> AAEPASRNVPFPYAETDVADLQARMTAGELDSTTLTQAYLQRIAALDRTGPRLHAVIELNPDALKEAAERDRERRDGRLRGPLHGIPLLLKDNINAAPMATSAGSLALQDFRPDDAYLVRRLRDAGAVVLGKTNLSEWMNFRSNNSISGWSARGGQTRNPYRPSHSPCGSSSGSAVAVAANLASVAIGTETDGSIVCPAAINGVVGLKPTVGLVSRDGI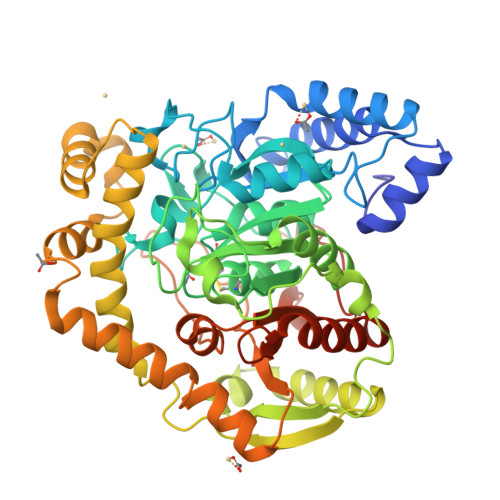IPISFSQDTPGPMARSVADAAAVLTAIAGRDPADPATATMPGRAVYDYTARLDPQGLRGKRIGLLQVPLLKYRGMPPLIEQAATELRRAGAVVVPVELPNYGAWAEAERTLLLYEFKAGLERYFNTHRAPLRSLADLIAFNQAHSKQELALFGQELLVEADATAGLADPAYIRARSDARRLAGPEGIDAALAAHQLDALVAPTTGVAWPIRPEGDDFPGESYSAAAVAGYPSLTVPMGQIDGLPVGLLFMGTAWSEPKLIEMAYAYEQRTRARRPPHFDTDALIDAGEPHHHHHH>MELPNIMHPVAKLSTALAAALMLSGCMPGEIRPTIGQQMETGDQRFGDLVFRQLAPNVWQHTSYLDMPGFGAVASNGLIVRDGGRVLVVDTAWTDDQTAQILNWIKQEINLPVALAVVTHAHQDKMGGMDALHAAGIATYANALSN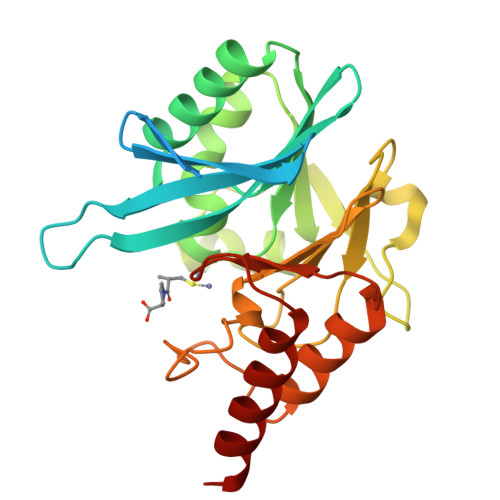QLAPQEGMVAAQHSLTFAANGWVEPATAPNFGPLKVFYPGPGHTSDNITVGIDGTDIAFGGCLIKDSKAKSLGNLGDADTEHYAASARAFGAAFPKASMIVMSHSAPDSRAAITHTARMADKLRLV[2x]>NLLRRSGKRRRSESGSDSFSGSGGDSSASPQFLSGSVLSPPPGLGRCLKAAAAGECKPTVPDYERDKLLLANWGLPKAVLEKYHSFGVKKMFEWQAECLLLGQVLEGKNLVYSAPTSAGKTLVAELLILKRVLEMRKKALFILPFVSVAKEKKYYLQSLFQEVGIKVDGYMGSTSPSRHFSSLDIAVCTIERANGLINRLIEENKMDLLGMVVVDELHMLGDSHRGYLLELLLTKICYITRKSASCQADLASSLSNAVQIVGMSATLPNLELVASWLNAELYHTDFRPVPLLESVKVGNSIYDSSMKLVREFEPMLQVKGDEDHVVSLCYETICDNHSVLLFCPSKKWCEKLADIIAREFYNLHHQAEGLVKPSECPPVILEQKELLEVMDQLRRLPSGLDSVLQKTVPWGVAFHHAGLTFEERDIIEGAFRQGLIRVLAATSTLSSGVNLPARRVIIRTPIFGGRPLDILTYKQMVGRAGRKGVDTVGESILICKNSEKSKGIALLQGSLKPVRSCLQRREGEEVTGSMIRAILEIIVGGVASTSQDMHTYAACTFLAASMKEGKQGIQRNQESVQLGAIEACVMWLLENEFIQSTEASDGTEGKVYHPTHLGSATLSSSLSPADTLDIFADLQRAMKGFVLENDLHILYLVTPMFEDWTTIDWY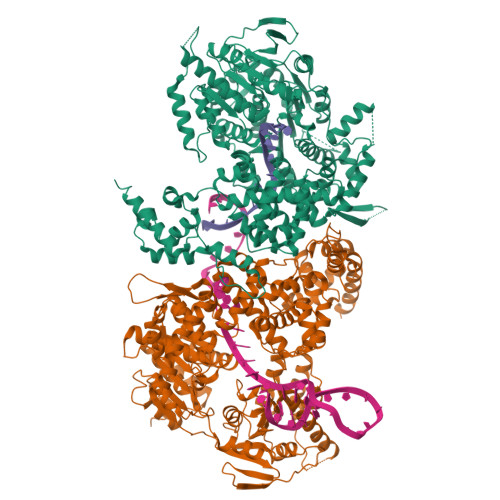RFFCLWEKLPTSMKRVAELVGVEEGFLARCVKGKVVARTERQHRQMAIHKRFFTSLVLLDLISEVPLREINQKYGCNRGQIQSLQQSAAVYAGMITVFSNRLGWHNMELLLSQFQKRLTFGIQRELCDLVRVSLLNAQRARVLYASGFHTVADLARANIVEVEVILKNAVPFKSARKAVDEEEEAVEERRNMRTIWVTGRKGLTEREAAALIVEEARMILQQDLVEM[2x]> TTKKRVFHFGKGKSEGNKTMKELLGGKGANLAEMASIGLSVPPGFTVSTEACQQYQDAGCALPAGLWAEIVDGLQWVEEYMGATLGDPQRPLLLSVRSGAAVSMPGMMDTVLNLGLNDEVAAGLAAKSGERFAYDSFRRFLDMFGNVVMDIPRSLFEEKLEHMKESKGLKNDTDLTASDLKELVGQYKEVYLSAKGEPFPSDPKKQLELAVLAVFNSWESPRAKKYRSINQITGLRGTAVNVQCMVFGNMGNTSGTGVLFTRNPNTGEKKLYGEFLVNAQGEDVVAGIRTPEDLDAMKNLMPQAYD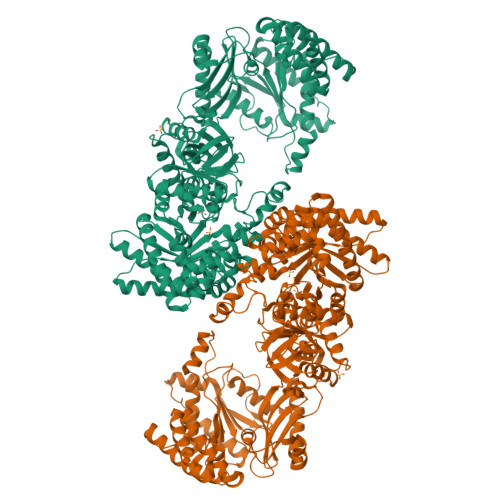ELVENCNILESHYKEMQDIEFTVQENRLWMLQCRTGKRTGKSAVKIAVDMVNEGLVEPRSAIKMVEPGHLDQLLHPQFENPSAYKDQVIATGLPASPGAAVGQVVFTAEDAEAWHSQGKAAILVRAETSPEDVGGMHAAVGILTERGGMTSHAAVVARGWGKCCVSGCSGIRVNDAEKLVTIGGHVLREGEWLSLNGSTGEVILGKQPLSPPALSGDLGTFMAWVDDVRKLKVLANADTPDDALTARNNGAQGIGLCRTEHMFFASDERIKAVRQMIMAPTLELRQQALDRLLPYQRSDFEGIFRAMDGLPVTIRLLDPPLHEFLPEGNIEDIVSELCAETGANQEDALARIEKLSEVNPMLGFRGCRLGISYPELTEMQARAIFEAAIAMTNQGVQVFPEIMVPLVGTPQELGHQVTLIRQVAEKVFANVGKTIGYKVGTMIEIPRAALVADEIAEQAEFFSFGTNDLTQMTFGYSRDDVGKFIPVYLAQGILQHDPFEVLDQRGVGELVKFATERGRKARPNLKVGICGEHGGEPSSVAFFAKAGLDYVSCSPFRVPIARLAAAQVLV>GSTPAAPLDVKCLEANKDYIIISWKQPAVDGGSPILGYFIDKCEVGTDSWSQCNDTPVKFARFPVTGLIEGRSYIFRVRAVNKMGIGFPSRVSEPVAALDPAEKARLKSRPS[4x]

Obscurin, or its homolog obscurin-like-1, bridges the giant ruler titin and the myosin crosslinker myomesin at the M-band. Myomesin is a 185 kDa modular protein that localizes exclusively at the M-band, where anti-parallel dimers cross link myosin filaments. In addition to a mechanical role, myomesin is also needed for the integration of obscurin and its smaller obscurin-like-1 homolog at the M-band (Fukuzawa et al., 2008). Yeast two-hybrid and biochemical analyses have mapped the obscurin/obscurin-like-1:myomesin interaction to the linker region (L) located between the fourth and fifth Fn-III domains of myomesin (My4 and My5, respectively) and the third Ig domain of either obscurin or obscurin-like-1 (O3 and OL3, respectively) (inset) (Fukuzawa et al., 2008).

The ability of OL3:My4L to transition from the solution conformation to that observed crystallographically suggests that the LH helix might have a degree of flexibility. We explored this by solving the crystal structure of My4LH (myomesin residues 510–618) in two different space groups (data collection and refinement statistics in Table 1). In space group P65 (2.05 Å resolution), all four My4LH independent molecules in the a.u. display clear electron density until residue A608, while residues E609-S618 (LH) cannot be modeled. The My4 domain displays the typical Fn-III fold made of seven anti-parallel β-strands organized in two separate β-sheets (A-B-E and C-C′-F-G) arranged in a β sandwich. Overall, SAXS and crystallographic analyses support a model in which interdomain freedom allows the transition from a relatively compact solution conformation to an open one that can be stabilized by homodimerization.> GPLGSEPRSLTAEEVKRLEEQEEDTFRELRIFLRNVTHRLAIDKRFRVFTKPVDPDEVPDYVTVIKQPMDLSSVISKIDLHKYLTVKDYLRDIDLICSNALEYNPDRDPGDRLIRHRACALRDTAYAIIKEELDEDFEQLAEEIQESRKKRG;> SGRGKGGKGLGKGGA

ATPase family, AAA domain-containing protein 2 (ATAD2), also known as ANCCA (AAA+ nuclear coregulator cancer-associated), has a bromodomain and two AAA ATPase domains. The ATAD2 bromodomain (BRD) contains the canonical, left-handed bundle structure of four α-helices (αZ, αA, αB, αC), which support the two highly variable loops, ZA (residues 1003–1030) and BC (residues 1063–1068), which are responsible for forming peptide docking sites. The bromodomain of the ATAD2 protein is classified as a family IV bromodomain based on conserved residues and the structural features it shares with other members of family IV. This chromatin binding protein is able to recognize acetylated lysine through its bromodomain, a chromatin reader domain that is highly conserved across species. ATAD2 was shown to recognize a di-acetylated histone H4K5acK12ac modification that is associated with newly synthesized histones.

To better understand how this longer BRD recognizes di-acetylated ligands, we grew crystals of the ATAD2 BRD (residues 966–1112, C1101A) in complex with the histone H4K5acK8ac (1–10) peptide. While there was missing electron density beyond ligand residue 7, we observed excellent density for residues Ser1-Lys5. Five polar contacts between the ligand and residues in the ATAD2 bromodomain are present in our structure. Y1063 is responsible for two of these contacts. It forms hydrogen bonds using its backbone carbonyl oxygen to the backbone amide of Gly2, and through its side chain hydroxyl group to the backbone amide of Gly4. As seen in other BRD structures, the conserved asparagine (N1064) coordinates the acetylation modification on residue K5ac. The carbonyl oxygen of the acetyl group is coordinated through hydrogen bonding with the side chain amide of N1064. It is also coordinated through an ordered water molecule at the base of the binding pocket that also interacts with Y1021. Members of the ZA loop, V1013, V1018, and the gatekeeper residue I1074 coordinate the acetyllysine residue, potentially by interacting with the carbon atoms in the side chain of K5ac in the binding pocket.> GPTVGGQLGTAGQGFSYSKSNGRGGSQAGGSGSAGQYGSDQQHHLGSGSGAGGTGGPAGQAGRGGAAGTAGVGETGSGDQAGGEGKHITVFKTYISPWERAMGVDPQQKMELGIDLLAYGAKAELPK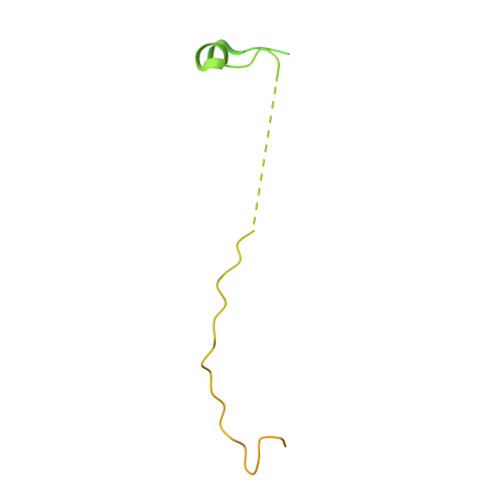YKSFNRTAMPYGGYEKASKRMTFQMPKFDLGPLLSEPLVLYNQNLSNRPSFNRTPIPWLSSGEPVDYNVDIGIPLDGETEEL>MRRVAVLGAGPSGLTAARYLKQAGFEVMVFERYHHVGGTWNYTDETWMSEDGRPVYSSMYQNLFVNLPKELMAFPDFPFHDIEGSYVPSKEVLKYFDNFTDAFDLRKLIKLQHHVENVRPCESGWLVTVTDLTTMVEHSFEFDAVVVCTGQTWCPLYPDVEGRSFFRGRLTHAHEFRSPEPFRNKRVLIVGAGPSGHDMALHISYVSKEVFLSRKELKPVEGLFPDNVTEKPLLTSLSEYTAHFSDGTSTDVDEILYCTGYRYRFPFLSPECGVTVDEKYVYPLYLHMLNINKPTMLFIGVSYNACYSIMFDLQAQWVTAVLAGR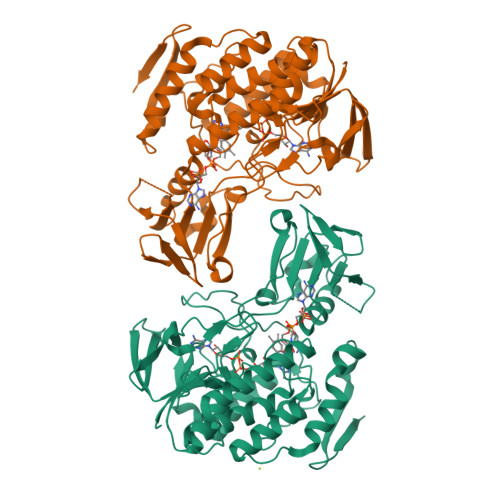CTLPDAETMRKEEAEYMEKQRAEAVHPHVLMNHQWEYFKKLEEMSGAKTMPPVYMKMFDDVASDLVKDLQNFRKNNYMIIDNENYKKIYAAALEHHHHHH[4x]> MSSDKNGDILRPLSDSEVDELLDLYKVKFGIRNFHYLLLYNQRKWDRQLSEAQIPRNDLNHISLRKQFYTHRRGNFRTWGTYVSLHRD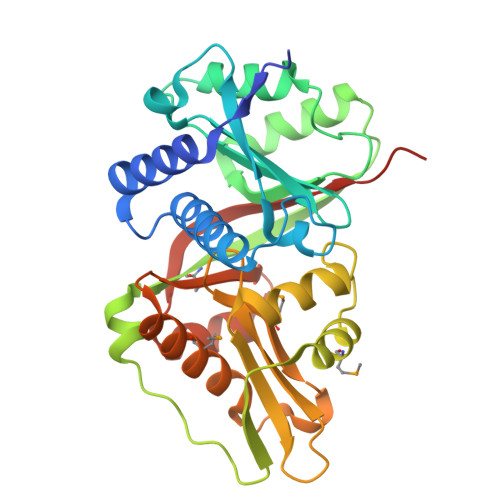IVQSVSFFSWQPDGAAELWECLEQTQLIEWTQGALLTNVDLGFCNRVKELAVSRGVTAIQPRQCFGMVLSHEDAFCAKVPDLPSEFEIRRLRAEDAAMVHDSWPNKGEGSLTYLQALVRFNKSLGICRSDTGELIAWIFQNDFSGLGMLQVLPKAERRGLGGLLAAAMSREIARGEEITLTAWIVATNWRSEALLKRIGYQKDLVNEWIKLVPNSSLEHHHHHH>[236x]XSKLLELLRKLSEAL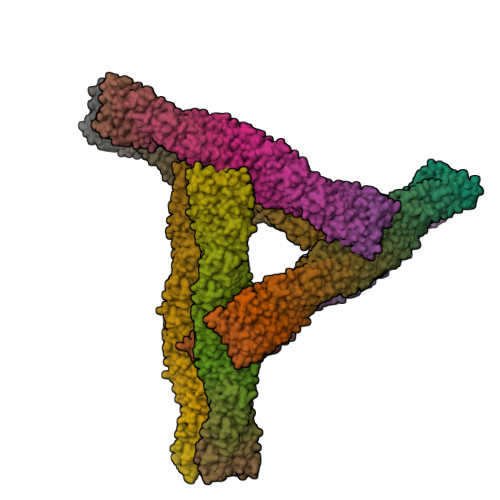HKAIELLEKWGX>QKPMYEVQWKVVEEINGNNYVYIDPTQLPYDHKWEFPRNRLSFGKTLGAGAFGKVVEATAYGLIKSDAAMTVAVKMLKPSAHLTEREALMSELKVLSYLGNHMNIVNLLGACTIGGPTLVITEYCCYGDLLNFLRRKRDSFICSKTSPAIMEDDELALDLED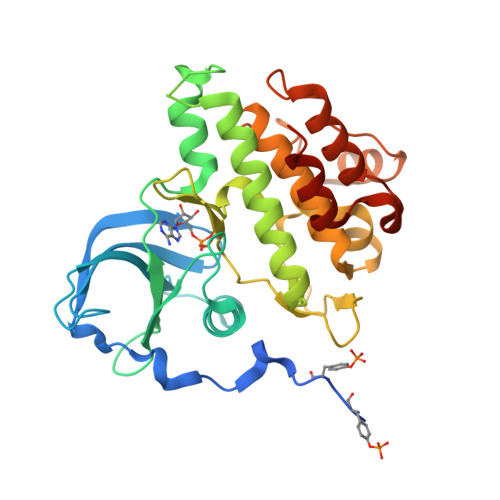LLSFSYQVAKGMAFLASKNCIHRDLAARNILLTHGRITKICDFGLARDIKNDSNYVVKGNARLPVKWMAPESIFNCVYTFESDVWSYGIFLWELFSLGSSPYPGMPVDSKFYKMIKEGFRMLSPEHAPAEMYDIMKTCWDADPLKRPTFKQIVQLIEKQISESTNHI[2x]>GHMNDLIDTTEMYLRTIYDLEEEGVVPLRARIAERLEQSGPTVSQTVARMERDGLLTVAEDRHLELTKAGRARAISVMRKHRLAERLLVDVIGLEWEQVHLEACRWEHVMSEAVERKLVKLLGNPTTSPYGNPIPGLDELGVGDSVEPVDTDLRRVDEVARSGGGRALVCRIAEHVQLDPDLMSELKKVGVVPGNEIDIVAVAGVNKPIQVQGSEGGTQLQPGIAHAVMVRVK[2x]

The iron-dependent regulator IdeR is the main transcriptional regulator controlling iron homeostasis genes in Actinobacteria, including species from the Corynebacterium, Mycobacterium and Streptomyces genera, as well as the erythromycin-producing bacterium Saccharopolyspora erythraea. IdeR is an OCS from the DtxR (Diphtheria toxin repressor) family of transcriptional regulators which typically consist of three domains: an N-terminal DNA-binding winged helix-turn-helix (wHTH) motif, followed by a dimerization interface that contains most of the metal-binding residues, and a C-terminal SH3-like domain (21–23). The main function of IdeR is to repress the expression of iron uptake genes when the intracellular iron levels are sufficient. When iron levels are sufficient for iron ions to occupy the IdeR metal-binding sites, the regulator is activated and recognizes a highly conserved 19-bp sequence located in the promoter region of its target genes.

We determined the crystal structure of Co2+-activated IdeR at 2.0 Å resolution. Each subunit consists of the three domains typical of an IdeR protein, an N-terminal domain containing the DNA-binding wHTH motif, a dimerization domain, and a C-terminal SH3-like domain. Two metal-binding sites are formed by residues from all three domains, coordinating two Co2+ ions in octahedral geometry. The overall structure of SeIdeR is highly similar to the structures of IdeR from M. tuberculosis and DtxR from C. diphtheriae. The structures of these IdeR dimers are very similar to the DNA-free dimer structure. DNA binding primarily causes a slight shift of the recognition helices, which is necessary to allow these helices to insert into the major grooves of the DNA.> MANELTWHDVLAEEKQQPYFLNTLQTVASERQSGVTIYPPQKDVFNAFRFTELGDVKVVILGQDPYHGPGQAHGLAFSVRPGIAIPPSLLNMYKELENTIPGFTRPNHGYLESWARQGVLLLNTVLTVRAGQAHSHASLGWET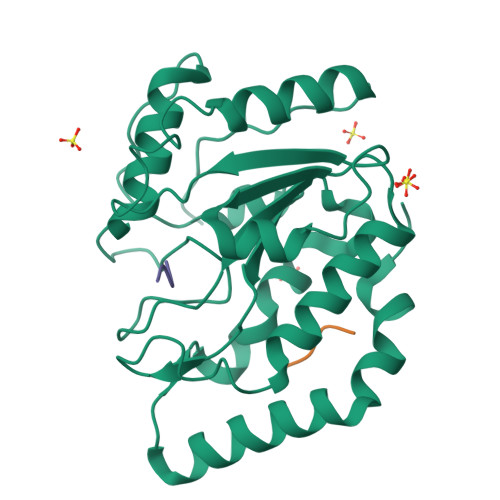FTDKVISLINQHREGVVFLLWGSHAQKKGAIIDKQRHHVLKAPHPSPLSAHRGFFGCNHFVLANQWLEQRGETPIDWMPVLPAESELEHHHHHH;>MDFDDDIPF[2x]>MATNAKPVYKRILLKLSGEALQGTEGFGIDASILDRMAQEIKELVELGIQVGVVIGGGNLFRGAGLAKAGMNRVVGDHMGMLATVMNGLAMRDALHRAYVNARLMSAIPLNGVCDSYSWAEAISLLRNNRVVILSAGTGNPFFTTDSAACLRGIEIEANVVLKATKVDGVFTADPAKDPTATMYEQLTYSEVLEKELKVMDLAAFTLARDHKLPIRVFNMNKPGALRRVVMGEKEGTLIT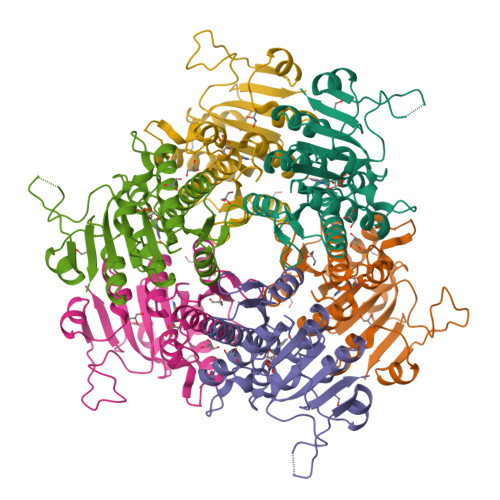E[2x]> MGRENVLPVHNDVYEDFVFTTPYFQPESTFKSVPKLFSDILLGGVEWVYTTSESVLAYDYKLWYLWSGVSNLDESFDMFFNQYWALSLSTSVFQLFYAVILDRYLSVLFQNTPYTNDWFRMMLHSKETALIWLYHPELSWHINGLNQFFTYFYGGILEFVYFDKSNPDMCILVHTLWIHLLILFLIFTGFVTILFSFYGNPNTEENTIDSDYLAASGTVEAEKEITSIDDYLGLVFAIAYVFGVFFYVHGWTSMLSHAVLLLS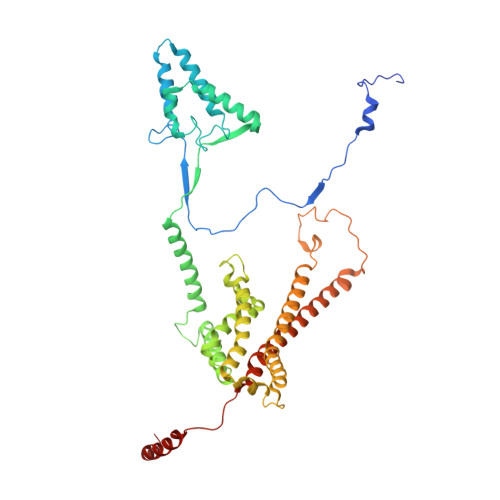CYSIIIMFLFILGMPTLLLYDFGIFFLAYLKGAGKYISSVAEMMFDYTACLVFYIRILAQWIRVVLMVVTFISLSHYVSDFDITNSALIGSENQSDSMNELNTNFSMTYYILTVLPGKFIYWIYEILHTFFVVCSQFVAFFAIVFWLFLFLYTFFIIEKHEDFFSKKREERKKKLKELWNLKN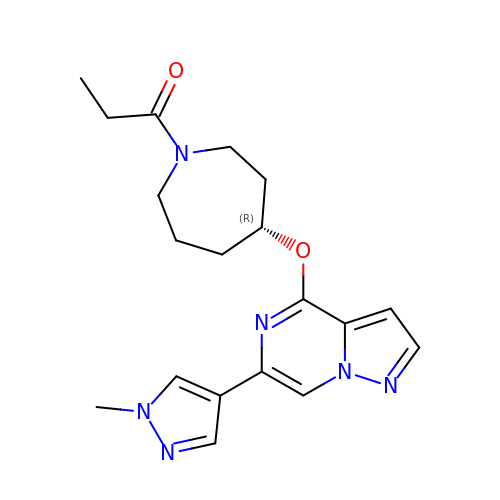1-[(4R)-4-{[(6P,8S)-6-(1-methyl-1H-pyrazol-4-yl)pyrazolo[1,5-a]pyrazin-4-yl]oxy}azepan-1-yl]propan-1-one | C19 H24 N6 O2 | ZGDYATLTXZZPSE-OAHLLOKOSA-N>[2x]GMTSPSIESGARERTRRAILDAAMLVLADHPTAALGDIAAAAGVGRSTVHRYYPERTD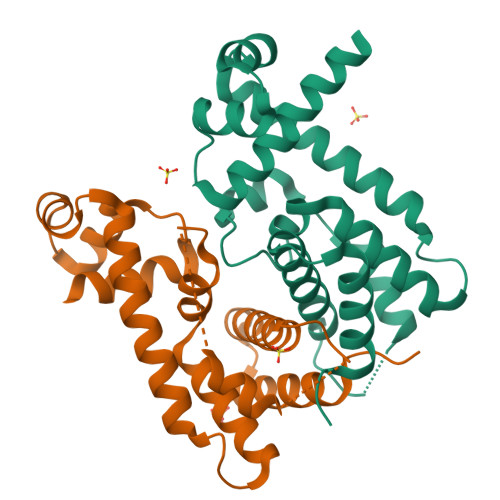LLRALARHVHDLSNAAIERADPTSGPVDAALRRVVESQLDLGPIVLFVYYEPSILADPELAAYFDIGDEAIVEVLNRASTERPEYPPGWARRVFWALMQAGYEAAKDGMPRHQIVDAIMTSLTSGIITLPRT> MGHHHHHHSYHDSIKDSIKAVVNISTEKKIKNNFIGGGVFNDPFFQQFFGDLGGMIPKERMERALGSGVIISKDGYIVTNNHVIDGADKIKVTIPGSNKEYSATLVGTDSESDLAVIRITKDNLPTIKFSDSNDISVGDLVFAIGNPFGVGESVTQGIVSALNKSGIGINSYENFIQTD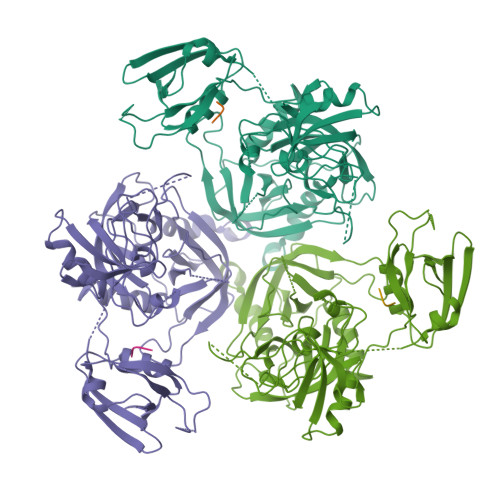ASINPGNSGGALIDSRGGLVGINTAIISKTGGNHGIGFAIPSNMVKDTVTQLIKTGKIERGYLGVGLQDLSGDLQNSYDNKEGAVVISVEKDSPAKKAGILVWDLITEVNGKKVKNTNELRNLIGSMLPNQRVTLKVIRDKKERAFTLTLAERKNPNKKETISAQNGAQGQLNGLQVEDLTQETKRSMRLSDDVQGVLVSQVNENSPAEQAGFRQGNIITKIEEVEVKSVADFNHALEKYKGKPKRFLVLDLNQGYRIILVK ARS2 is a direct interaction partner of CBC and together they form a platform for the assembly of co-transcriptional complexes that determine the fate of diverse RNA Pol II transcripts. Our structural analysis shows that ARS2 is made up of two regions, residues 147–270 and 408–763 that co-fold into a structured core with an intervening glutamate-rich region of unknown function that is likely unstructured. The human ARS2 core has an unusual structure comprising a largely helical ‘body’ from which project N- and C-terminal ‘legs’. We find that the RRM domain is required to bind RNA, whereas a basic patch in the C-terminal leg of ARS2 mediates the interaction with FLASH.

Based on this model, additional constructs for crystallisation were designed in which disordered loops A (538–552) and B (568–598) were truncated. Crystals of ARS2147–270+408–763Δ568–598 (Δloop B) diffracted to 3.37 Å resolution (space group C2221) and exhibited an ordered loop A. A composite model, including both loop A (from the ARS2147–270+408–763Δ568–598 structure) and most of loop B (from the ARS2147–270+408–763 structure) was artificially constructed and used for illustrative purposes since it is almost complete, only lacking residues 578–598. In mammals, loop A (538-ASEPGT543PPLPTSLPS-552) is highly conserved and proline-rich. In most crystal forms, the loop is disordered presumably due to flexibility. However, in the crystal form in which loop B (see below) was deleted, loop A is well structured in one monomer, likely due to crystal-packing constraints. Interestingly, T543 is a major phosphorylation site of human ARS2 (Discussion). Loop B (residues 566–598) is around 30-residues long in metazoans, half the length in S. pombe and absent in plants. In metazoans, the first part of the loop is highly acidic (566-EEVSAEEEELLG-577), whereas the second half of the loop is proline-rich, particularly in mammals. Elution from the resin shows that ARS2147–871, as well as various loop-deletion constructs used for crystallisation (ARS2171–270+408–763, ARS2147–270+408–763ΔloopB and ARS2171–270+408–763ΔloopAΔloopB) are all retained by the NCBP3 bound to the resin. Nevertheless, despite extensive co-crystallisation trials, including with the loop B/‘EEEE’ helix deletion mutant, we have never observed any electron density corresponding to FARB bound to ARS2 in a crystal, and all our biochemical evidence suggests that only the C-terminal foot is involved.

>PVMKTFKEFLLSLDDSVDETEAVKRYNDYKLDFRRQQMQDFFLAHKDEEWFRSKYHPDEVGKRRQEARGALQNRLRVFLSLMETGWFDNLLLDIDKADAIVKMLDAAVIKMEGGTENDLRILEQ[2x];>[2x]GLECKPRPLHKTCSLFMRNIAPNISRAEIISLCKRYPGFMRVALSEPQPERRFFRRGWVTFDRSVNIKEICWNLQNIRLRECELSPGVNRDLTRRVRNINGITQHKQIVRNDIKLAAKLIHTLDDRTQLWASEPGTPPLPTSLPSQNPILKNITDYLIEEGSGSGSERDEKLIKVLDKLLLYLRIVHSLDYYNTCEYPNEDEMPNRCGIIHVRGPMPPNRISHGEVLEWQKTFEEKLTPLLSVRESLSEEEAQKMGRKDPEQEVEKFVTSNTQELGKDKWLCPLSGKKFKGPEFVRKHIFNKHAEKIEEVKKEVAFFNNFLTDAKRPALPE>STPSIVIASAARTAVGSFNGAFANTPAHELGATVISAVLERAGVAAGEVNEVILGQVLPAGEGQNPARQAAMKAGVPQEATAWGMNQLC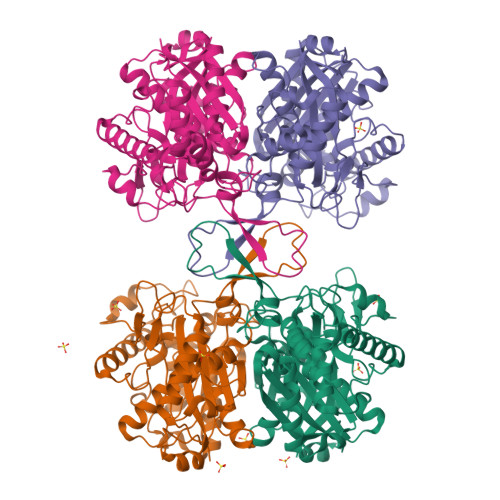GSGLRAVALGMQQIATGDASIIVAGGMESMSMAPHCAHLRGGVKMGDFKMIDTMIKDGLTDAFYGYHMGTTAENVAKQWQLSRDEQDAFAVASQNKAEAAQKDGRFKDEIVPFIVKGRKGDITVDADEYIRHGATLDSMAKLRPAFDKEGTVTAGNASGLNDGAAAALLMSEAEASRRGIQPLGRIVSWATVGVDPKVMGTGPIPASRKALERAGWKIGDLDLVEAHEAFAAQACAVNKDLGWDPSIVNVNGGAIAIGHPIGASGARILNTLLFEMKRRGARKGLATLCIGGGMGVAMCIESL[4x]> DANLLNDRVLRAMLKAEETCAPSVSYFKCVQKEVLPSMRKIVATWMLEVCEEQKCEEEVFPLAMNYLDRFLSLEPVKKSRLQLLGATCMFVASKMKETIPLTAEKLCIYTDNSIRPEELLQMELLLVNKLKWNLAAMTPHDFIEHFLSKMPEAEENKQIIRKHAQTFVALCATDVKFISNPPSMVAAGSVVAAVQGLNLRSPNNFLSYYRLTRFLSRVIKCDPDCLRACQEQIEALLESSLRQAQQNMD;> GEFATSRYEPVAEIGVGAYGTVYKARDPHSGHFVALKSVRVPNGEEGLPISTVREVALLRRLEAFEHPNVVRLMDVCATSRTDREIKVTLVFEHVDQDLRTYLDKAPPPGLPAETIKDLMRQFLRGLDFLHANCIVHRDLKPENILVTSGGTVKLADFGLARIYSYQMALTPVVVTLWYRAPEVLLQSTYATPVDMWSVGCIFAEMFRRKPLFCGNSEADQLGKIFDLIGLPPEDDWPRDVSLPRGAFPPRGPRPVQSVVPEMEESGAQLLLEML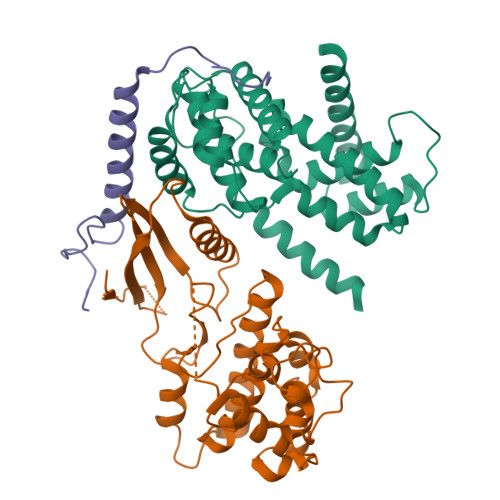TFNPHKRISAFRALQHSYLHKDEGNPE;> GEFRQNPCGSKACRRLFGPVDSEQLSRDCDALMAGCIQEARERWNFDFVTETPLEGDFAWERVRGLGLPKLYLPTGPRRG> MEPAGRFTKVAAAVADSVVTIESVSDQEGMQGSGVIVDGRGYIVTNNHVISEAANNPSQFKTTVVFNDGKEVPANLVGRDPKTDLAVLKVDNVDNLTVARLGDSSKVRVGDEVLAVGAPLGLRSTVTQGIVSALHRPVPLSGEGSDTDTVIDAIQTDASINHGNSGGPLIDMDAQVIGINTAGKSLSDSASGLGFAIPVNEMKLVANSLIKDGKIVHPTLGIS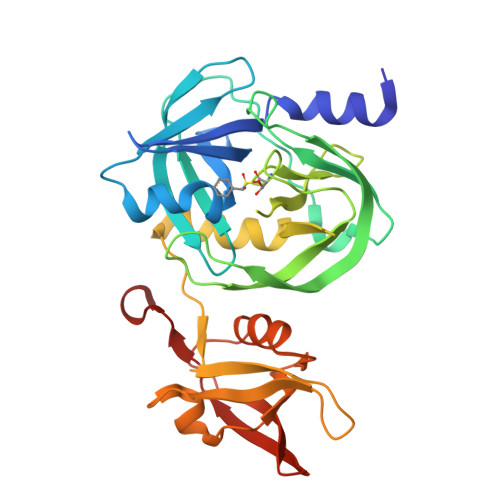TRSVSNAIASGAQVANVKAGSPAQKGGILENDVIVKVGNRAVADSDEFVVAVRQLAIGQDAPIEVVREGRHVTLTVKPDPDSTLEHHHHHH> SPSAEECGYSDRVRSMTLGNSTITTQESANVVVGYGEWPSYLSDREATAEDQPTQPDVATCRFYTLESVQWEKTSPGWWWKFPEALKNMGLFGQNMHYHYLGRAGYTIHVQCNASKFHQGCLLVVCVPEAEMGCADTDTTFPATELTTEDTPHVFTSDSITGKKVQAAVCNAGMGVGVGNLTIFPHQWINLRTNNSATIVIPYINSVPMDNMFRHYNFTLMIIPFAPL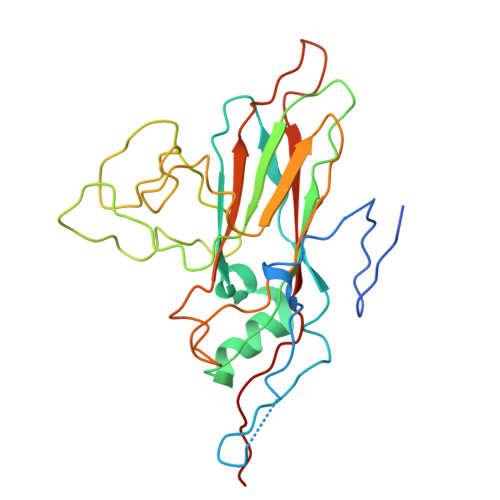NFTDGATAYVPITVTIAPMYAEYNGLRLASTQ> EELYQSILELKPLTLLMTSSTSFSETINQWADILKTTDMEKFSFDSNPINLLELVKQFNLYVDELAITCEANNVWAKERIDSTPNLFALYDNSGGEAIHGHAFVPYYKESIVLRRLFTVDPNTFNLSRFAAFEGPCQLYCAAHADSAWVKIQTLLTLGNGIINTLKIIKQAQAFGIDEAVTENLKALKEQFIAFQLAEADIKESLKAPSFAEPLPNKESEFFYPIDEKALAKMNGYQLATICL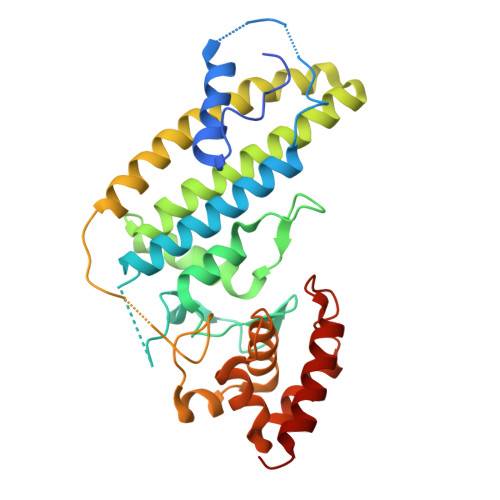EELNSPKPSPLIERILSNKKFWKRINSAFESGVFKGRTDDPAGKIAKIREWHQLLQISG> MKFGLFFLNFMNSKRSSDQVIEEMLDTAHYVDQLKFDTLAVYENHFSNNGVVGAPLTVAGFLLGMTKNAKVASLNHVITTHHPVRVAEEACLLDQMSEGRFAFGFSDCEKSADMRFFNRPTDSQFQLFSECHKIINDAFTTGYCHPNNDFYSFPKISVNPHAFTEGGPAQFVNATSKEVVEWAAKLGLPLV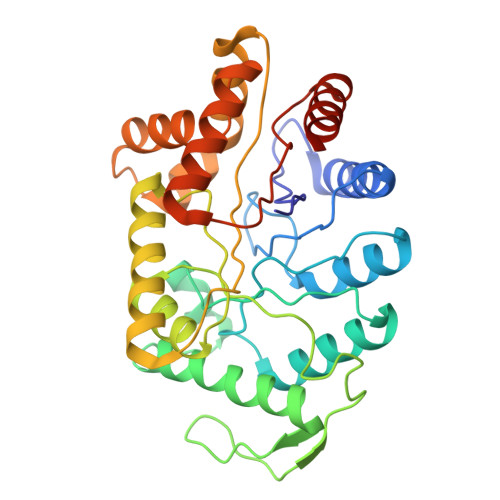FRWDDSNAQRKEYAGLYHEVAQAHGVDVSQVRHKLTLLVNQNVDGEAARAEARVYLEEFVRESYSNTDFEQKMGELLSENAIGTYEESTQAARVAIECCGAADLLMSFESMEDKAQQRAVIDVVNANIVKYHS> MRLTKFTDLALRSLMRLAVVRDGDEPLATREVAEVVGVPYTHAAKAITRLQHLGVVEARRGRGGGLTLTDLGRRVSVGWLVRELEGEAEVVDCEGDNPCPLRGACRLRRALRDAQEAFYAALDPLTVTDLVAAPTGPVLLGLTDRPSGKLAAALEHHHHHH

The most widespread dedicated NO sensor regulator in bacteria is NsrR, a member of the Rrf2 superfamily of homodimeric transcriptional regulators. NsrR proteins from Bacillus subtilis (Bs) and Streptomyces coelicolor (Sc) have been shown to bind a [4Fe–4S] cluster, which functions as the NO sensing module34. In ScNsrR, reaction with NO was shown to result in loss of the iron–sulfur (Fe–S) cluster and formation of iron-nitrosyl species. This process led to loss of high affinity DNA-binding and activation of genes that were previously repressed by [4Fe–4S] (holo-)ScNsrR, including those encoding Hmp-type NO detoxifying enzymes.

We report here the 1.95 Å resolution crystal structure of holo-ScNsrR, the first for an Fe–S cluster-bound form of any Rrf2 superfamily regulator. ScNsrR crystallized as a dimer spanning a distance of about 80 Å, with monomers being related by a crystallographic twofold axis. Nevertheless, the polypeptide chain was resolved for 137 of its 148 amino acid residues and forms two loosely interacting domains (residues 1–85 and 86–144, see Methods section). Another similarity to other Rrf2 superfamily members is the highly hydrophobic nature of the ScNsrR dimerization interface, which buries a surface of about 2,050 Å2 per monomer. Unique to the holo-ScNsrR structure is the presence of a [4Fe–4S] cluster that is ligated by three cysteine residues (Cys93, Cys99 and Cys105) from one monomer and Asp8 from the other. The latter forms a salt bridge with Arg12 from the same α1 helix, which also interacts with the carbonyl oxygen of Val36 of the DNA-binding helix-turn-helix (HTH) motif. At the opposite side of the cluster Cys93 is exposed to solvent. The more buried Cys99 and Cys105 Sγ atoms are hydrogen-bonded to the main chain N atoms of Leu101 and Arg108, respectively. Otherwise, the cluster environment is mainly hydrophobic, without H-bonds to the inorganic S atoms of the cluster. Holo-ScNsrR appears to be the first structurally characterized protein with a [4Fe–4S] cluster that is asymmetrically bound by ligands from two different subunits as indicated by our examination of all the other [4Fe–4S] cluster-containing protein structures found in the Protein Data Bank18.>[2x]TTHLVWFRQDLRLHDNLA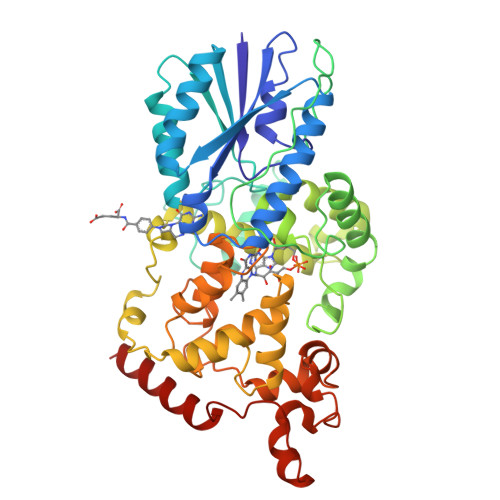LAAACRNSSARVLALYIATPRQWATHNMSPRQAELINAQLNGLQIALAEKGIPLLFREVDDFVASVEIVKQVCAENSVTHLFYNYQYEVNERARDVEVERALRNVVCEGFDDSVILPPGAVMTGNHEMYKVFTPFKNAWLKRLREGMPECVAAPKVRSSGSIEPSPSITLNYPRQSFDTAHFPVEEKAAIAQLRQFCQNGAGEYEQQRDFPAVEGTSRLSASLATGGLSPRQCLHRLLAEQPQALDGGAGSVWLNELIWREFYRHLITYHPSLCKHRPFIAWTDRVQWQSNPAHLQAWQEGKTGYPIVDAAMRQLNSTGWMHNRLRMITASFLVKDLLIDWREGERYFMSQLIDGDLAANNGGWQWAASTGTDAAPYFRIFNPTTQGEKFDHEGEFIRQWLPELRDVPGKVVHEPWKWAQKAGVTLDYPQPIVEHKEARVQTLAAYEAARKGK> MTNWESLYEKALDKVEASIRKVRGVLLAYNTNIDAIKYLKREDLEKRIEKVGKEEVLRYSEELPKEIETIPQLLGSILWSIKRGKAAELLVVSREVREYMRKWGWDELRMGGQVGIMANLLGGVYGIPVIAHVPQLSELQASLFLDGPIYVPTFERGELRLIHPREFRKGEEDCIHYIYEFPRNFKVLDFEAPRENRFIGAADDYNPILYVREEWIERFEEIAKRSELAIISGLHPLTQENHGKPIKLVREHLKILNDLGIRAHLEFAFTPDEVVRLEIVKLLKHFYSVGLNEVELASVVSVMGEKELAERIISKDPADPIAVIEGLLKLIKETGVKRIHFHTYGYYLALTREKGEHVRDALLFSALAAATKAMKGNIEKLSDIREGLAVPIGEQGLEVEKILEKEFSLRDGIGSIEDYQLTFIPTKVVKKPK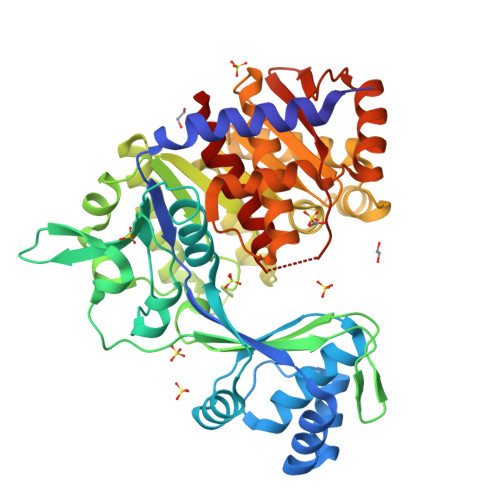STVGIGDTISSSAFVSEFSLH>MPYEWENPQLVSEGTEKSHASFIPYLDPFSGEWEYPEEFISLNGNWRFLFAKNPFEVPEDFFSEKFDDSNWDEIEVPSNWEMKGYGKPIYTNVVYPFEPNPPFVPKDDNPTGVYRRWIEIPEDWFKKEIFLHFEGVRSFFYLWVNGKKIGFSKDSCTPAEFRLTDVLRPGKNLITVEVLKWSDGSYLEDQDMWWFAGIYRDVYLYALPKFHIRDVFVRTDLDENYRNGKIFLDVEMRNLGEEEEKDLEVTLITPDGDEKTLVKETVKPEDRVLSFAFDVKDPKKWSAETPHLYVLKLKLGEDEKKVNFGFRKIEIKDGTLLFNGKPLYIKGVNRHEFDPDRGHAVTVERMIQDIKLMKQHNINTVRTSHYPNQTKWYDLCDYFGLYVIDEANIESHGIDWDPEVTLANRWEWEKAHFDRIKRMVERDKNHPSIIFWSLGNEAGDGVNFEKAALWIKKRDNTRLIHYEGTTRRGESYYVDVFSLMYPKMDILLEYASKKREKPFIMCEYAHAMGNSVGNLKDYWDVIEKYPYLHGGCIWDWVDQGIRKKDENGREFWAYGGDFGDTPNDGNFCINGVVLPDRTPEPELYEVKKVYQNVKIRQVSKDTYEVENRYLFTNLEMFDGAWKIRKDGEVIEEKTFKIFAEPGEKRLLKIPLPEMDDSEYFLEISFSLSEDTPWAEKGHVVAWEQFLLKAPAFEKKSISDGVSLREDGKHLTVEAKDTVY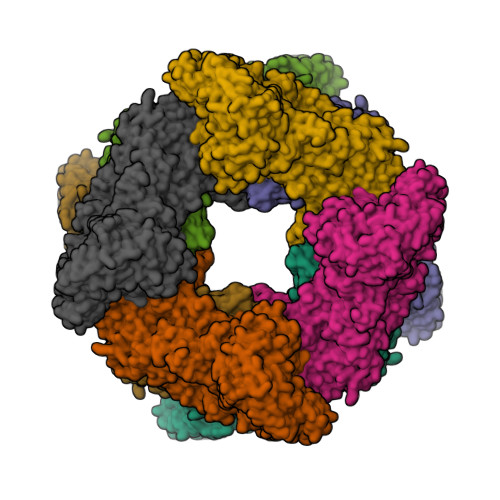VFSKLTGLLEQILHRRKKILKSPVVPNFWRVPTDNDIGNRMPQRLAIWKRASKERKLFKMHWKKEENRVSVHSVFQLPGNSWVYTTYTVFGNGDVLVDLSLIPAEDVPEIPRIGFQFTVPEEFGTVEWYGRGPHETYWDRKESGLFARYRKAVGEMMHRYVRPQETGNRSDVRWFALSDGETKLFVSGMPQIDFSVWPFSMEDLERVQHISELPERDFVTVNVDFRQMGLGGDDSWGAMPHLEYRLLPKPYRFSFRMRISEEIPSWRVLAAIPETLHVEMSSEDVIREGDTLRVKFSLLNDTPLSKEKQVVLFVDGNEYSVRRVVIPPFKKEELVFKVEGLKKGEHLIHTNLNTRKTIYVR[4x]>[2x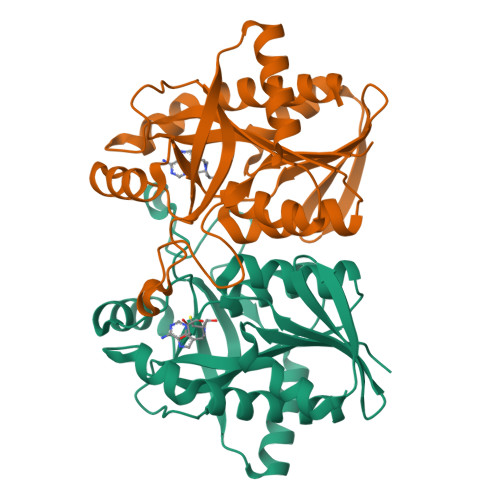]MGHHHHHHSGMKIAILGAMSEEITPLLETLKDYTKIEHANNTYYFAKYKDHELVLAYSKIGKVNSTLSASVMIEKFGAQVLLFTGVAGAFNPELEIGDLLYATKLAQYDLDITAFGHPLGFVPGNEIFIKTDEKLNNLALEVAKELNIKLRAGIIATGDEFICDEAKKAKIREIFNADACEMEGASVALVCDALKVPCFILRAMSDKAGEKAEFDFDEFVINSAKISANFVLKMCEKL Mutations in dysferlin, the first protein linked with the cell membrane repair mechanism, causes a group of muscular dystrophies called dysferlinopathies. Dysferlin, a member of the ferlin protein family, is a type II anchored membrane protein with a single C terminal helix buried in the membrane. Dysferlin is not a part of the dystrophin-glycoprotein complex, but its function is linked with calcium-activated membrane repair caused by fusing aggregated intracellular vesicles with the sarcolemma at the site of injury. One DysF domain is inserted into the other DysF domain, by gene duplication, forming an inner DysF domain and a two part (N terminal and C terminal) outer DysF domain.

A single dataset was collected in a different space group P212121 (orthorhombic) to 2.2 Å. The crystal packing is almost the same in the two forms, but the distortions of the perfect cube in the orthorhombic structure means the monomers of the crystallographic trimer in the cubic crystals are no longer identical. This leads to some of the flexible regions (eg residues 965-671) being more visible in some chains with the orthorhombic data. The structure is highly conserved between independent copies in the crystals. The crystallographic trimer of the P213 crystal superimposes onto the trimer in the P212121 asymmetric unit with an RMSD Calpha of 0.89 Å over 326 residues of the trimer. The four individual chains from the two assymetric units superimpose no worse than 0.79 Å Calpha RMSD over 108 residues for any pair. The biggest variation between dysferlin models is between 965 and 971 and 1018 and 1021. These are also the regions with the highest temperature (B) factors in dysferlin, the regions with the largest RMS between NMR models in myoferlin, as can be seen from the CING database, and the regions that differ most between dysferlin and myoferlin. The trimer (with 9 phosphates) is predicted to be the stable assembly by PDBePISA. We have no evidence from gel filtration or NMR spectroscopy (data not shown) for the existence of a trimer, nor is there any likely way to invoke a trimer in vivo.

>[3x]SMDAGHLSFVEEVFENQTRLPGGQWIYMSDNYTDVNGEKVLPKDDIECPLGWKWEDEEWSTDLNRAVDEQGWEYSITIPPERKPKHWVPAEKMYYTHRRRRWVRLRRRDLSQ> MKKVCFVCLGNICRSPMAEFVMKSIVSSDVMMIESRATSDWEHGNPIHSGTQSILKTYQINYDITKCSKQITITDFNTFDYIIGMDSDNVKNLKEMSQHQWDSKIYL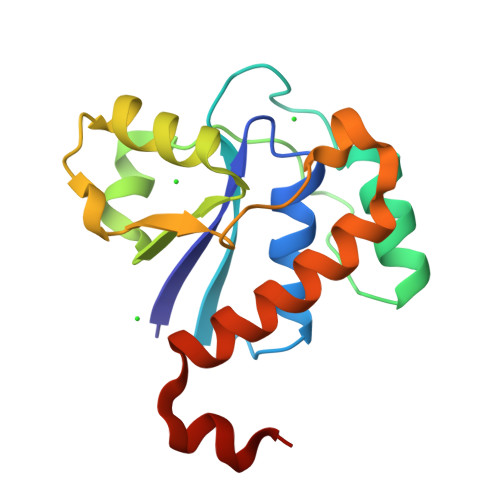FREGGVPDPWYTNDFEETYQLVRKGCQDWLSRLMSKEYLEHHHHHH~{N}-[(4~{R})-4-cyclohexyl-2,5-bis(oxidanylidene)imidazolidin-1-yl]-4,5,6,7-tetrakis(fluoranyl)-1~{H}-indole-3-carboxamide 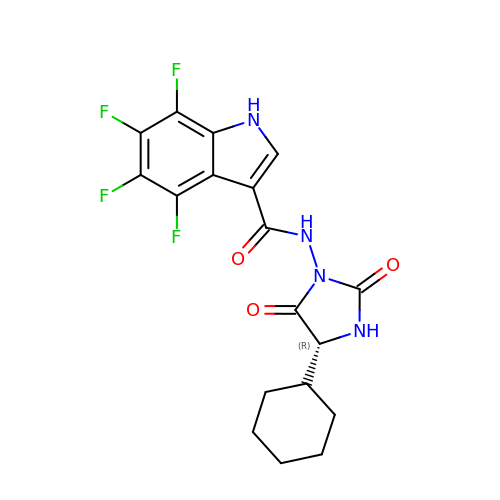| C18 H16 F4 N4 O3 | PPXDFGIAKBMPEQ-CQSZACIVSA-N> STKCVTIPTEMAMCNDVGYSEMRLPNLMGHTNMAEVVPKSAEWQNLLQTGCHPYARTFLCSLFAPVCLDTFIQPCRSMCVAVRDSCAPVLACHGHSWPESL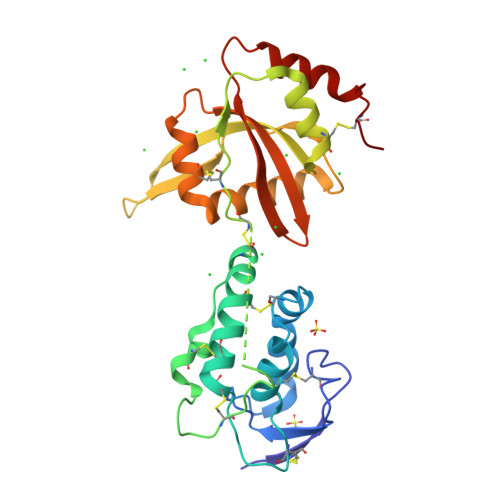DCDRFPAGEDMCLDTLSKEYQYSYKELPKPSCQGCPLIEEFFSHKTVLEAFCDNNFAVKVKLAKKKSASGLYEYETEGPVEFIKQGLLLPYDTRTMIEQWLLINENCAQKLIRTRPTVYVIAGEIHHGKVKVNRIFHWQKKDSQLTLATRRWRHHKCAAA> MSAPAAAPKHPG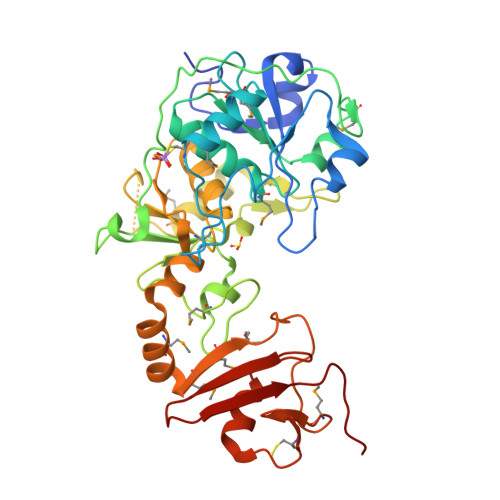KVFLDPSEVADHLAEYRIVDCRYSLKIKDHGSIQYAKEHVKSAIRADVDTNLSKLVPTSTARHPLPPCAEFIDWCMANGMAGELPVLCYDDECGAMGGCRLWWMLNSLGADAYVINGGFQACKAAGLEMESGEPSSLPRPATHWPFKTAFQHHYLVDEIPPQAIITDARSADRFASTVRPYAADKMPGHIEGARNLPYTSHLVTRGDGKVLRSEEEIRHNIMTVVQGAGDAADLSSFVFSCGSGVTACINIALVHHLGLGHPYLYCGSWSEYSGLFRPPIMRSIIDDYGMCMQMQTPSLGDNPKANLDTMTLKVDGAPCERPDAEVQSAATHLHAGEAATVYFKSGRVVTIEVPVVPNLEA> SGAGICS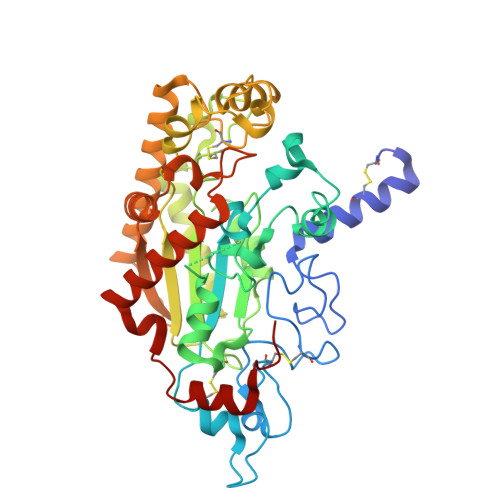LPFLAKICQKIKLAIKNSVPIKDVDSDKYSIFPTLRGYHWRGRDCNDSDKTVYPGRRPDNWDAHRDSNCNGIWGVDPKDGIPYEKKFCEGSQPRGIILLGDAAGAHFHIPPEWLTVSQMSVNSFLNLPTAVTNELDWPQLSGTTGFLDSASKIKENSIYLRLRKRNRCNHRDYQNISKNGASSRNVKSLIESLSRNQLLDHPAIVIYAMIGNDVCNGRKTDPVSAMTTPEQLYANVLKMLEALNSHLPTGSHVILYGLAHGAFLWDTLHSRYHPLGQLNKDVTYTQLYSFLGCLQVSPCPGWMSANETLRALTSERAQQLSETLRKIAASKKFTNFNLFYLDFAFQEVVEEWQKMGGQPWELIEAVDGFHPNEVALLLFADQLWEKVQRQWPDVLGKENPFNPQIEEVFGDQGGH>[4x]MHHHHHHSSGMSDKIIHLTDDSFDTDVLKADGAILVDFWAEWCGPCKMIAPILDEIADEYQGKLTVAKLNIDQNPGTAPKYGIRGIPTLLLFKN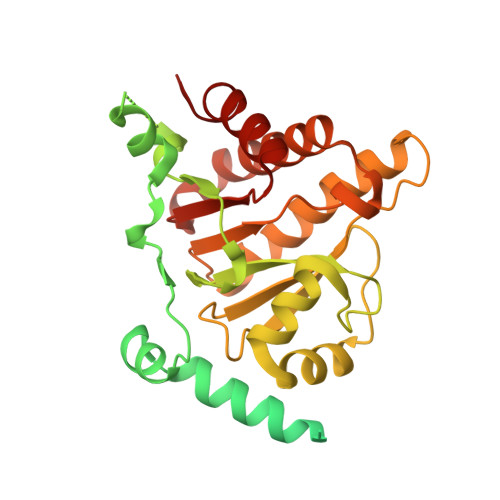GEVAATKVGALSKGQLKEFLDANLAGTENLYFQSMKKKVWREEKERLLKMTLEERRKEYLRDYIPLNSILSWKEEMKGKGQNDEENTQETSQVKKSLTEKVSLYRGDITLLEVDAIVNAANASLLGGGGVDGCIHRAAGPCLLAECRNLNGCDTGHAKITCGYDLPAKYVIHTVGPIARGHINGSHKEDLANCYKSSLKLVKENNIRSVAFPCISTGIYGFPNEPAAVIALNTIKEWLAKNHHEVDRIIFCVFLEVDFKIYKKKMNEFFSVD>GSHMSDSNTITSFQVDCYLWHIRKLLSMRDMCDAPFDDRLRRDQKALKGRGSTLGLDLRVATMEGKKIVEDI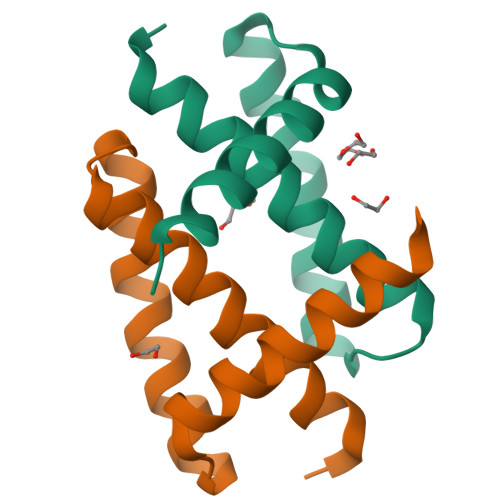LKSET[2x]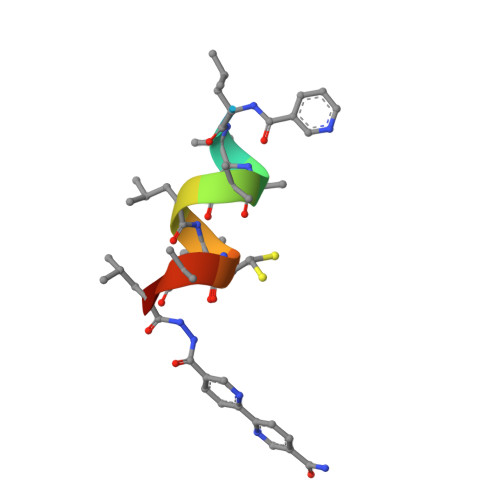> XLAAALACALX N-[3-(N'-HYDROXYCARBOXAMIDO)-2-(2-METHYLPROPYL)-PROPANOYL]-O-TYROSINE-N-METHYLAMIDE 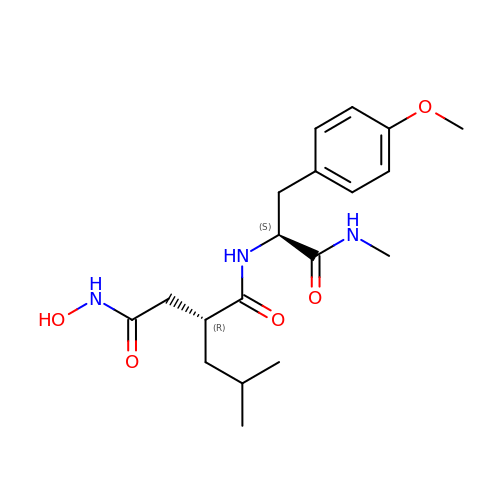| C19 H29 N3 O5 | QYZPDCGWIJYZMN-ZBFHGGJFSA-N> GDICIKDSINTLWTGIKPPPNCQIVENTDTNDGKLTLVLVKNGGLVNGYVSLVGVSDTVNQMFTQKSATIQLRLYFDSSGNLLTDESNLKIPLKNKSSTATSEAATSSKAFMPSTTAYPFNTTTRDSENYIHGICYYMTSYDRSLVPLNISIMLNSRTISSNVAYAIQFEWNLNAK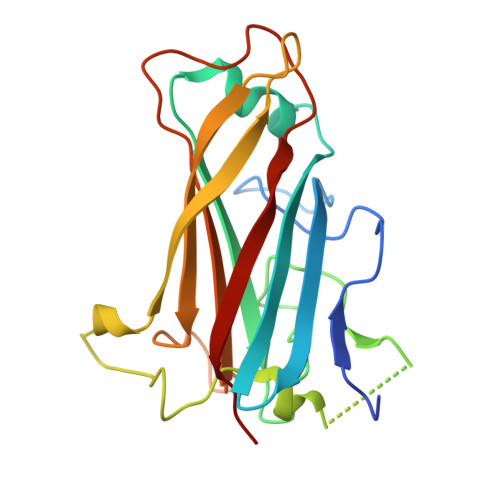ESPESNIATLTTSPFFFSYIREDDN> MSENTVMPIVRVAVLAAGDDGGRLTEMALPSELPLREILPAVQRIVQPARENDGAADPAAAPNPVRLSLAPIGGAPFSLDATLDTVGVVDGDLLALQAVPSGPPAPRIVEDIADAAVIFSEARR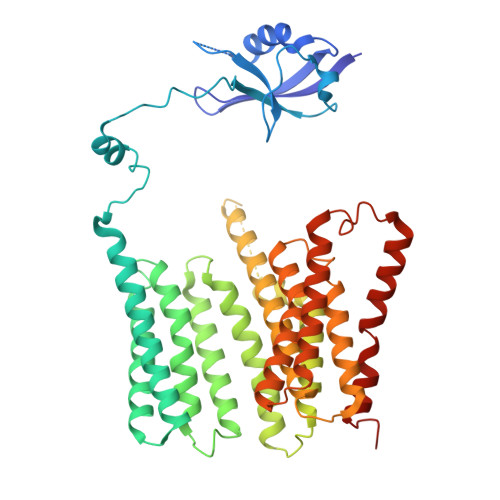RQWGPTHIARGAALALIGLILVGTGLSVAHRVITGDLLGQFIVSGIALATVIAALAVRNRSAVLATSLAVTALVPVAAAFALGVPGDFGAPNVLLAAAGVAAWSLISMAGSPDDRGIAVFTATAVTGVGVLLVAGAASLWVISSDVIGCALVLLGLIVTVQAAQLSAMWARFPLPVIPAPGDPTPAARPLSVLADLPRRVRVSQAHQTGVIAAGVLLGVAGSVALVSSANASPWAWYIVVAAAAGAALRARVWDSAACKAWLLGHSYLLAVALLVAFVIGDRYQAALWALAALAVLVLVWIVAALNPKIASPDTYSLPMRRMVGFLATGLDASLIPVMALLVGLFSLVLDR>[8x]IVPTRELENVFLGRCKDYEITRYLDILPRVRSDCSALWKDFFKAFSFKNPCDLDLGSYKDFFTSAQQQLPKNKVMFWSGVYDEAHDYANT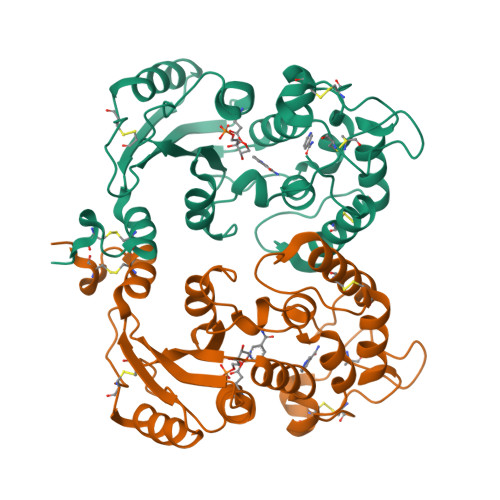GRKYITLEDTLPGYMLNSLVWCGQRANPGFNEKVCPDFKTCPVQARESFWGMASSSYAHSAEGEVTYMVDGSNPKVPAYRPDSFFGKYELPNLTNKVTRVKVIVLHRLGEKIIEKCGAGSLLDLEKLVKAKHFAFDCVENPRAVLFLLCSDNPNARECRLAKRFYRIA> STGEPAPVLSSPPPADVSTFLAFPSPEKLLRLGPKSSVLIAQQTDTSDPEKVVSAFLKVSSVFKDEATVRMAVQDAVDALMQKAFNSSSFNSNTFLTRLLVHMGLLKSEDKVKAIANL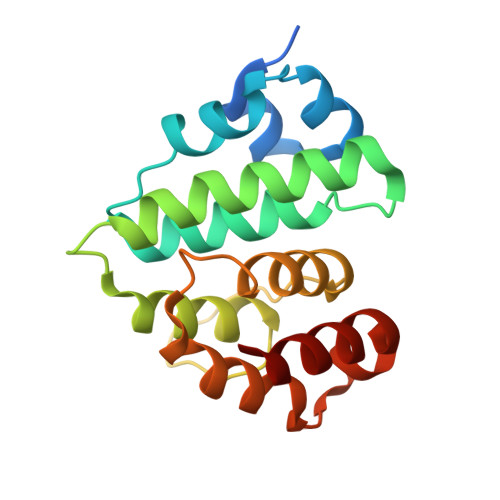YGPLMALNHMVQQDYFPKALAPLLLAFVTKPNSALESCSFARHSLLQTLYKV>MTSLFTTADHYHTPLGPDGTPHAFFEALRDEAETTPIGWSEAYGGHWVVAGYKEIQAVIQNTKAFSNKGVTFPRFETGEFELMMAGQDDPVHKKYRQLVAKPFSPEATDLFTEQLRQSTNDLIDARIELGEGDAATWLANEIPARLTAILLGLPPEDGDTYRRWVWAITHVENPEEGAEIFAELVAHARTLIAERRTNPGNDIMSRVIMSKIDGESLSEDDLIGFFTILLLGGIDNTARFLSSVFWRLAWDIELRRRLIAHPELIPNAVDELLRFYGPAMVGRLVTQEVTVGDITMKPGQTAMLWFPIASRDRSAFDSPDNIVIERTPNRHLSLGHGIHRCLGAHLIRVEARV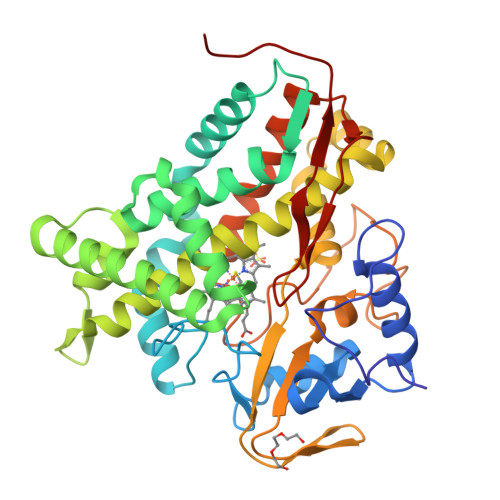AITEFLKRIPEFSLDPNKECEWLMGQVAGMLHVPIIFPKGKRLSE[2x]>[2x]GAMGSDFLLGNPFSSPVGQRIEKATDGSLQSEDWALNMEICDIINETEEGPKDALRAVKKRIVGNKNFHEVMLALTVLETCVKNCGHRFHVLVASQDFVESVLVRTILP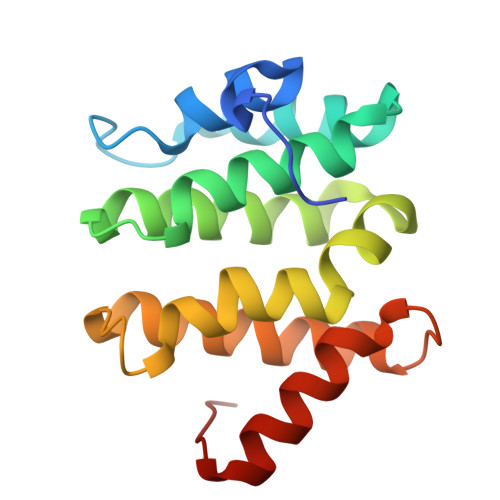KNNPPTIVHDKVLNLIQSWADAFRSSPDLTGVVTIYEDLRRKGLEFPM>MAHHHHHHMHLLDTLAEGLKEIDARGLRRRRRTADTPCAAHMTVDGRAIIGFASNDYLGLAAHPQLIAAIAEGAQRYGAGSGGSHLLGGHSRAHAQLEDDLAEFVGGFVENARALYFSTGYMANLATLTALAGRGTTLFSDALNHASLIDGARLSRADVQIYPHCDTDALSAMLEASDADVKVIVSDTVFSMDGDIAPLPRLLELAEQHGAWLIVDDAHGFGVLGPQGRGAIAQAALRSPNLISIGTLDKAAGVSGAFVAAHETVIEWLVQRARPYIFTTASVPAAAHAVSASLRIIGG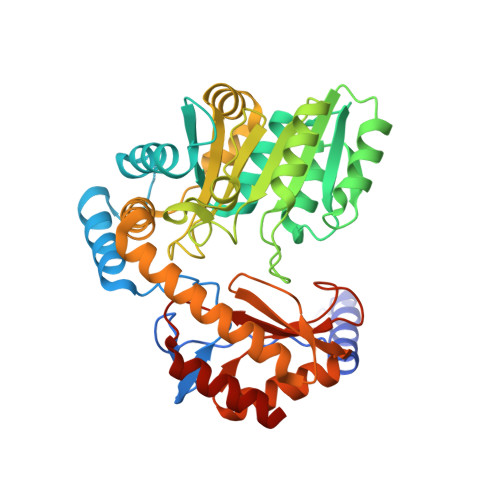EEGDARRAHLQQLIGRTRAMLKATPWLPVDSHTAVQPLIIGANDATLEIAATLDRAGLWVPAIRPPTVPTGTSRLRISLSAAHSQADLDRLEAGLQQLGAKAA[2x]>[8x]MSRVPSPPPPAEMSSGPVAESWCYTQIKVVKFSYMWTINNFSFCREEMGEVIKSSTFSSGANDKLKWCLRVNPKGLDEESKDYLSLYLLLVSCPKSEVRAKFKFSILNAKGEETKAMESQRAYRFVQGKDWGFKKFIRRDFLLDEANGLLPDDKLTLFCEVSVVQDSVNISGQNTMNMVKVPECRLADELGGLWENSRFTDCCL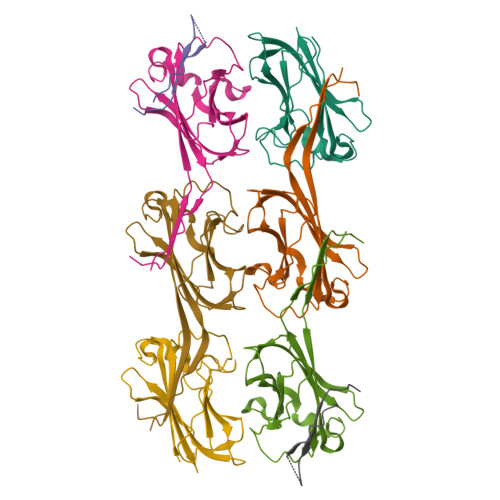CVAGQEFQAHKAILAARSPVFSAMFEHEMEESKKNRVEINDVEPEVFKEMMCFIYTGKAPNLDKMADDLLAAADKYALERLKVMCEDALCSNLSVENAAEILILADLHSADQLKTQAVDFINYHASDVLETSGWKSMVVSHPHLVAEAYRSLASAQCPFLGPPRKRLKQ>MDNVLLSGQTLHADHSLQAGAYTLTIQNKCNLVKYQNGRQIWASNTDRRGSGCRLTLLSDGNLVIYDHNNNDVWGSACWGDNGKYALVLQKDGRFVIYGPVLWSLGPNG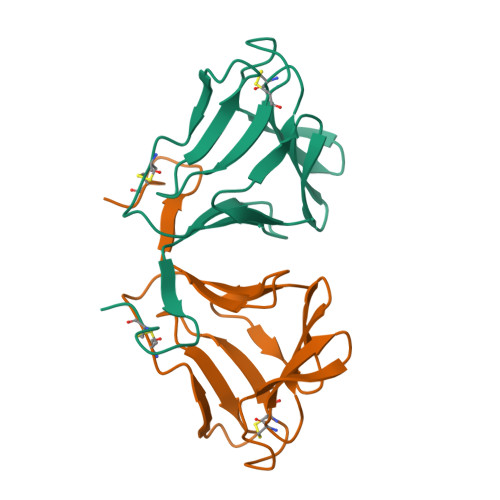CRRVNG[4x]> GAGCAGACATGACGACACTCA;> AGTCA;> TCTGAGTGC;> TGTCTGC

In this work, we exhaustively probe the ability of all 36 immobile HJ sequences to form DNA crystals in two different designed systems. Three separate self-assembling DNA crystal systems are described in this report: the “4 × 5” and “4 × 6” designs (collectively referred to as the 4 × N systems), and a third construct with a “scrambled” sequence variant of the 4 × 6 lattices. Self-assembly was mediated by three constituent oligonucleotides: (S1) containing four sequence repeats of either 5 or 6 bases; (S2) composed of 21 bases containing complementary regions to both (S1); and (S3) which forms the second junction crossover. The HJ serves as the fundamental component at the core of each unit, and the ultimate assembly of the full lattice is facilitated by the complementary 2-base sticky ends that tail each duplex.

The 4 × 5 system robustly crystallized with 75% of the junctions, and we obtained crystals in all but 9 of 36 sequences. Of the resulting structures, 18 exhibited P32 symmetry with average cell dimensions a = b = 68.85 Å c = 60.09 Å, with only nine retaining the original P3221 symmetry with average cell edges a = b = 68.17 Å c = 60.60 Å. Although the cell parameters between the two symmetries were virtually indistinguishable, the differences between the periodicity of the lattices is dramatic, with vastly different cavity sizes. While the highest resolution achieved for the J1 system was 3.1 Å, in roughly half of the crystals measured the resolutions were 3.05 Å or better, and as high as 2.9 Å (J6) and 2.75 Å (J19), for the P32 and P3221 symmetries, respectively. Pos1 and 2 were readily observable in the electron density maps at either one or both of these conserved sites in a significant number of the structures, with no apparent respect to motif or symmetry. However, in the majority of the crystal structures reported here, the cacodylate anion indeed fits best into the electron density map of our X-ray structures, due to the presence of sodium cacodylate in the crystallization solution.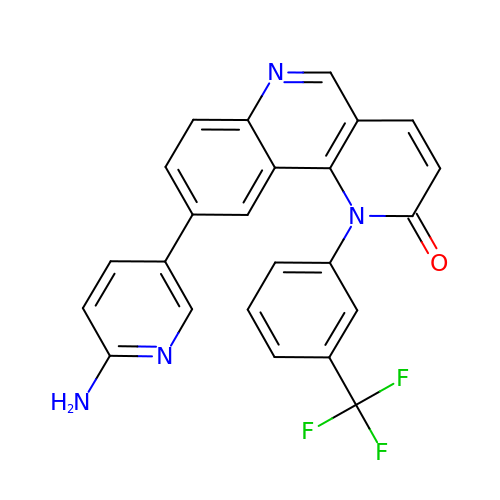9-(6-aminopyridin-3-yl)-1-[3-(trifluoromethyl)phenyl]benzo[h][1,6]naphthyridin-2(1H)-one | C24 H15 F3 N4 O | GUXXEUUYCAYESJ-UHFFFAOYSA-N SQT is one of many engineered protein scaffolds: it is based on human stefin A (SteA, also known as cystatin A) that has three possible insertion sites for peptides, namely the N-terminus, loop 1 (L1) and loop 2 (L2). Here we have used an SQT variant, named SQT-1C, with AU1 and Myc peptides inserted into loops L1 and L2, respectively, as a model to understand the effect of inserted peptides on scaffold structure, stability and oligomerisation properties. We show that inserted peptide regions play a crucial role in scaffold protein oligomerisation via domain swapping, leading to significantly different conformations and surface exposure of these binding epitopes in monomeric, dimeric and tetrameric forms.

SQT-1C crystallised only from the freshly-purified tetrameric fraction and in the presence of 19% dioxane, surprisingly yielding monomeric structure, which was solved to 2.5 Å resolution. X-ray crystallography confirmed that monomeric SQT-1C exhibits typical cystatin fold but only in very specific conditions, when crystallised in the presence of 19% dioxane. Interpretable electron density was observed for polypeptide regions R4-L48 and A93-N113 whilst residues D49-F75 were visible but less well ordered, indicating higher flexibility of this region. The SQT-1C monomer exhibits a cystatin-like architecture with five anti-parallel β-sheets and a perpendicular α-helix, showing that peptide insertions into loop regions do not affect the SQT scaffold backbone. The crystal structure reflects the dynamic nature of SQT-1C with higher than average B factors and less than ideal geometries. However, despite these shortcomings, the backbone fold and lattice interactions can be confidently discerned and have been extensively validated. SQT-1C oligomerisation state in solution under crystallisation conditions was further assessed by SEC, which revealed that in the presence of 19% dioxane SQT-1C is monomeric. However, in solution and in the absence of dioxane, monomeric SQT-1C exists in dynamic equilibrium with domain-swapped dimeric and dominant tetrameric species. To assess whether SQT-1C dimer models are consistent with the electron density observed in the crystal, we attempted to superimpose the DS SQT-1C homology model onto the SQT-1C crystal lattice. However, such a model was clearly incompatible with the packing observed in the crystalline lattice, encroaching into two of the symmetry related molecules, in agreement with SQT-1C being monomeric in the crystal state. Melting temperature of SQT-1C was 54 °C ± 1 °C, as measured by changes in intrinsic fluorescence, compared to 79.9 °C reported for SQT alone, which indicated that the inserted peptides significantly destabilized the scaffold.

> MIPRGLSEAKPATPEIQEIVDKVKPQLEEKTNETYGKLEAVQYKTQVLDTYRYILASTNYYIKVRAGDNKYMHLKVFNGPEQKLISEEDLADRVLTGYQVDKNKDDELTGFENLYFQSLERYLEHHHHHH> FMVSLPRMVYPQPKVLTPCRKDVLVVTPWLAPIVWEGTFNIDILNEQFRLQNTTIGLTVFAIKKYVAFLKLFLETAEKHFMVGHRVHYYVFTDQPAAVPRVTLGTGRQLSVLEVRAYKRWQDVSMRRMEMISDFCERRFLSEVDYLVCVDVDMEFRDHVGVEILTPLFGTLHPGFYGSSREAFTYERRPQSQAYIPKDEGDFYYLGGFFG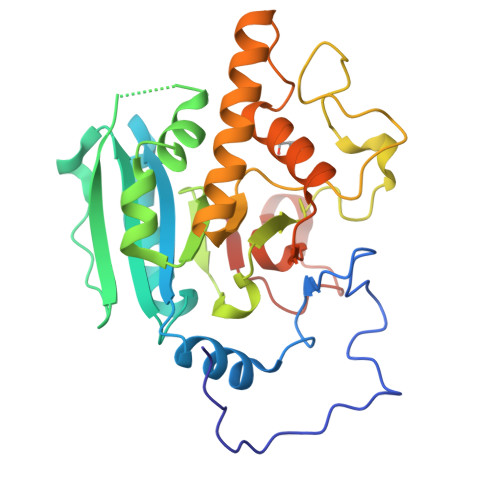GSVQEVQRLTRACHQAMMVDQANGIEAVWHCESHLNKYLLRHKPTKVLSPEYLWDQQLLGWPAVLRKLRFTAVPKNHQAVRNPE>[2x]MEVVAVHVIPRPHVNVDAALPLGRTPGMDKSAGSGSGSADA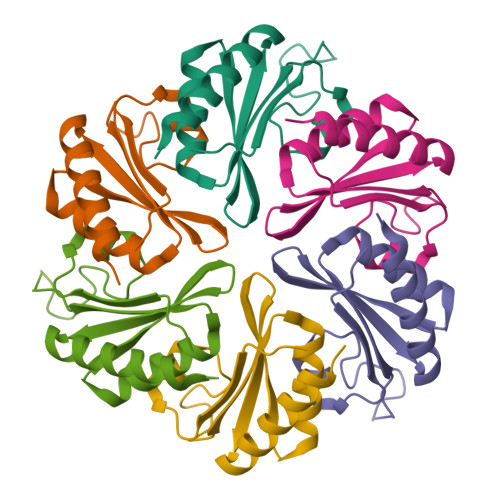LGMIEVRGFVGMVEAADAMVKAAKVELIGYEKTGGGYVTAVVRGDVAAVKAATEAGQRAAERVG6-[4-[[2,3-bis(chloranyl)phenyl]sulfonylamino]phenyl]-~{N}-[(3~{R})-pyrrolidin-3-yl]-2~{H}-pyrazolo[3,4-b]pyridine-4-carboxamide 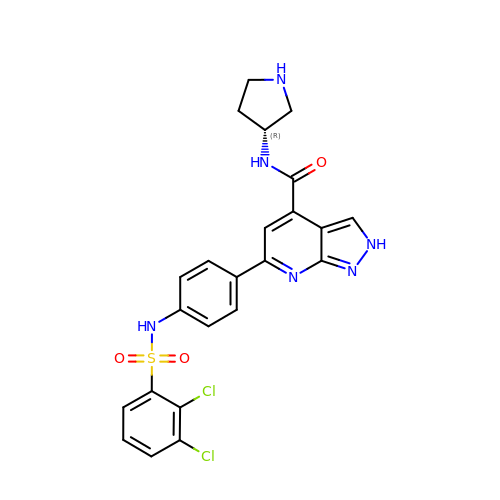| C23 H20 Cl2 N6 O3 S | UKMBVWVIQHGQEM-OAHLLOKOSA-N> MASMTGGQQMGRDEAGITGTWYNQLGSTFIVTAGADGALTGTYESAAGKAESRYVLTGRYDSAPATDGSGTALGWTVAWKNNYRNA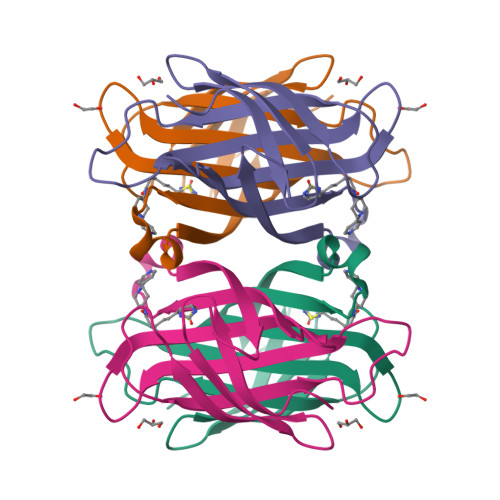HSATTWSGQYVGGAEARINTQWLLTAGATEANGWASTLVGHDTFTKVKPSAASIDAAKKAGVNNGNPLDAVQQ>[8x]MDDRLFRNAMGKFATGVTVITTELNGAVHGMTANAFMSVSLNPKLVLVSIGEKA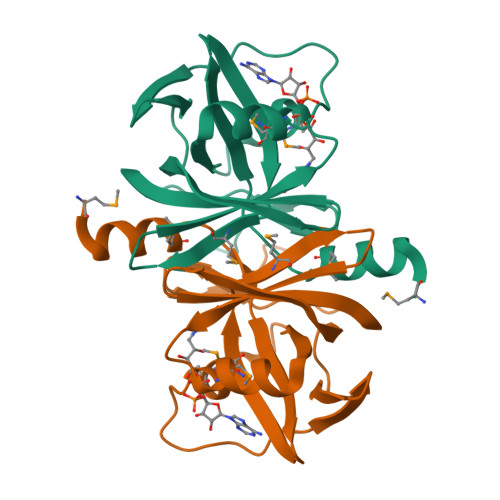KMLEKIQQSKKYAVNILSQDQKVLSMNFAGQLEKPVDVQFEELGGLPVIKDALAQISCQVVNEVQAGDHTLFIGEVTDIKITEQDPLLFFSGKYHQLAQNEKVETSS N-ethyl-4-{[(furan-2-yl)methyl]amino}-2-methyl-N-[(3S)-piperidin-3-yl]pyrimidine-5-carboxamide 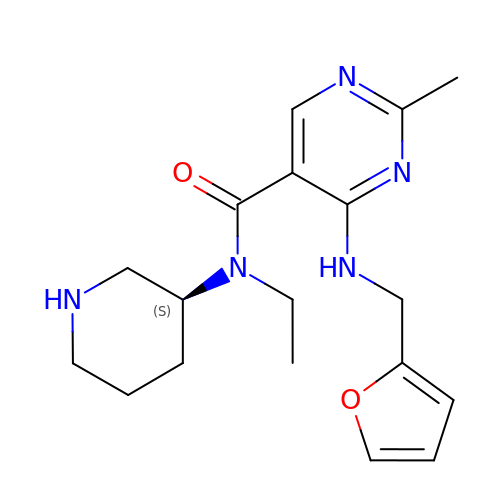| C18 H25 N5 O2 | GCBMAJYEAKERQU-AWEZNQCLSA-N>[4x]QSRGEKRTAHNAIEKRYRSSINDKIIELKDLVVGTEAKLNKSAVLRKAID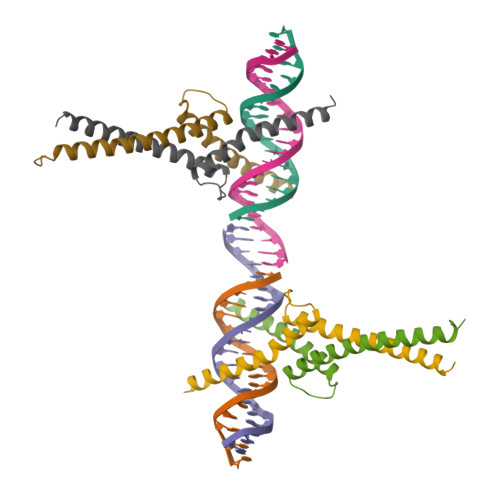YIRFLQHSNQKLKQENLSLRTAVHKSKSLKDL> MASSRRESINPWILTGFADAEGSFGLYIYNRNRGRIRYTTRLRFTITLHNKD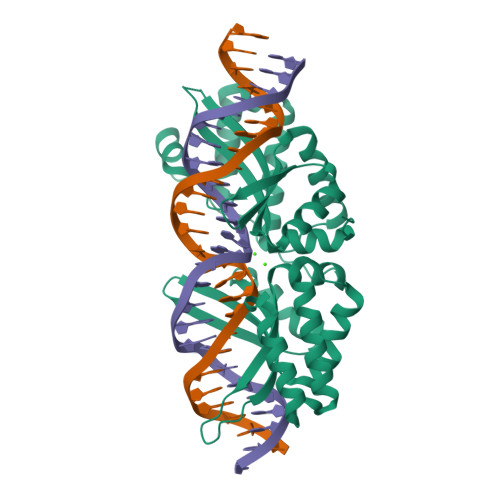KSILENIQSTWKVGIITNNGDNAVSLHVSRFEDLKVIIDHFEKYPLITQKLGDYKLFKQAFSVMENKEHLKENGIKELVRIKAKMNWGLTDELKKAFPGNISRERPLINKNIPNFKWLAGFTSGEGHFGVELIKNSRNSRVHVRLRFEIAQHVRDKNLMNSLITYLGCGYIYEQNYSERSWLRFSVSKFSDINDKIIPVFQENTLIGVKLEDFEDWCKVAKLIEEKKHLTESGLDEIKKIKLNMNKGR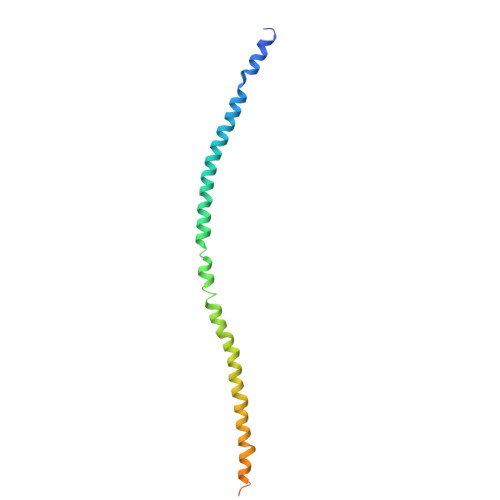> MVWDRQRLEKELEEKKEALELAIDQASRDYHRATALEKELEEKKKALELAIDQASQDYNRANVLEKELEAITREQEINRNLLGNAKLELDQLSSEKEQLTIEKAKLEEEKQISDASRQSLRRDLDASREAKKQVEKDLLEHHHHHH>LSTWQTFRRLWPTIAPFKAGLIVAGIALILNAASDTFMLSLLKPLLDDGFGATDRSVLLWMPLVVIGLMILRGITSYISSYCISWVSGKVVMTMRRRLFGHMMGMPVAFFDKQSTGTLLSRITYDSEQVASSSSGALITVVREGASIIGLFIMMFYYSWQLSIILVVLAPIVSIAIRVVSKRFRSISKNMQNTMGQVTTSAEQMLKGHKEVLIFGGQEVETKRFDKVSNKMRLQGMKMVSASSISDPIIQLIASLALAFVLYAASFPSVMDSLTAGTITVVFSSMIALMRPLKSLTNVNAQFQRGMAACQTLFAILDSEQEKDEGKRVIDRATGDLEFRNVTFTYPGREVPALRNINLKIPAGKTVALVGRSGSGKSTIASLITRFYDIDEGHILMDGHDLREYTLASLRNQVALVSQNVHLFNDTVANNIAYARTEEYSREQIEEAARMAYAMDFINKMDNGLDTIIGENGVLLSGGQRQRIAIARALLRDSPILILDEATSALDTESERAIQAALDELQKNRTSLVIAHRLSTIEQADEIVVVE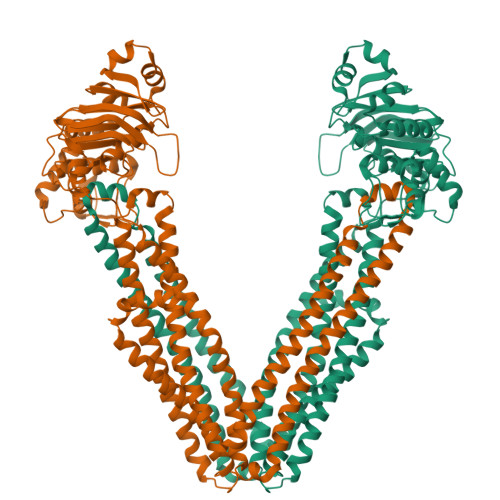DGIIVERGTHSELLAQHGVYAQLHKMQFGQ[2x]> FACKTANGTAIPIGGGSANVYVNLAPAVNVGQNLVVDLSTQIFCHNDYPETITDYVTLQRGSAYGGVLSSFSGTVKYNGSSYPFPTTSETPRVVYNSRTDKPWPVALYLTPVSSAGGVAIKAGSLIAVLILRQTNNYNSDDFQFVWNIYANNDVVVPTGGCDVSARDVTVTLPDYPGSVPIPLTVYCAKSQNLGYYLSGTTADAGNSIFTNTASFSPAQGVGVQLTRNGTIIPANNTVSLGAVGTSAV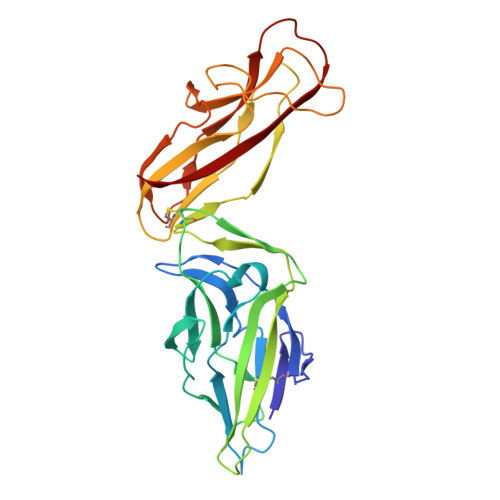SLGLTANYARTGGQVTAGNVQSIIGVTFVYQ> MGDQPFIPPPQQTALTVNDHDEVTVWNAAPCPMLPRDQVYVRVEAVAINPSDTKMRGQFATPWAFLGTDYAGTVVAVGSDVTHIQVGDRVYGAQNEMCPRTPDQGAFSQYTVTRGRVWAKIPKGLSFEQAAALPAGISTAGLAMKLLGLPLPSPSADQPPTHSKPVYVLVYGGSTATATVTMQMLRLSGYIPIATCSPHNFDLAKSRGAEEVFDYRAPNLAQTIRTYTKNNLRYALDCITNVESTTFCFAAIGRAGGHYVSLNPFPEHAATRKMVTTDWTLGPTIFGEGSTWPAPYGRPGSEEERQFGEDLWRIAGQLVEDG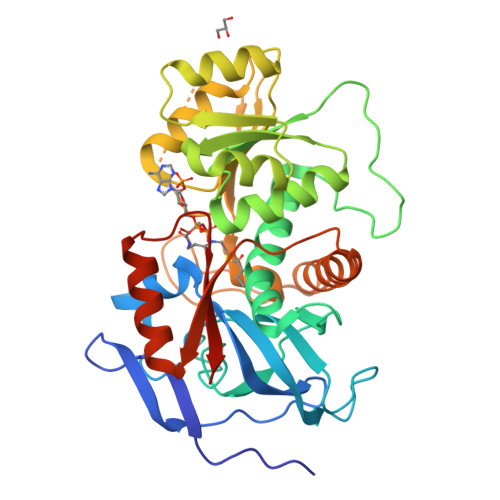RLVHHPLRVVQGGFDHIKQGMELVRKGELSGEKLVVRLEGPLEHHHHHH Leucyl-tRNA synthetases (LeuRSs) are examples of aaRSs that rely on their editing domains to limit misaminoacylation of tRNA with near-cognate amino acids and maintain the fidelity of the genetic code. Here, we identified epetraborole (EPT) from the MMV pandemic response box as an inhibitor against the essential protein leucyl-tRNA synthetase (LeuRS) in M. abscessus. Benzoxaboroles were shown to inhibit LeuRS in fungi, gram-negative pathogens and most recently M. tuberculosis. To gain insight into the interactions between EPT and LeuRS, we solved the crystal structure of the M. abscessus editing domain (LeuRS303-498).

AMP acts as a surrogate for the 3’ end of the tRNA acceptor stem. In concordance with the binding mode of action of benzoxaboroles, we detected strong electron density in the active site corresponding to the EPT-AMP adduct formed through covalent interactions between the boron atom of EPT and the 2’ and 3’ hydroxyl groups on the ribose ring of AMP. In addition, R435 (R449 in M. tuberculosis) hydrogen bonds with the ethoxy oxygen of EPT and packed with the ribose of AMP. EPT has a hydroxypropyl ether moiety, rather than the ethyl ether in the benzoxaborole bound to M. tuberculosis LeuRS, but the extension shows very weak electron density and likely does not contribute to binding. The only notable difference is a ~1 Å shift in phosphate group of the EPT-AMP adduct. In both complexes, the phosphate is pinned between Y421 (Y435) and T323 (T337). The electron density indicates that there are multiple rotomeric conformations of T323, meaning its hydroxyl could hydrogen bond with the phosphate or with the 3’ O and ether oxygen of the adduct. Comparing unliganded and liganded residues in M. abscessus editing domain structures shows a sizable shift of residues 416–422, located around the adenosine pocket, upon drug binding, including ordering of Y421 to interact with the EPT-AMP adduct phosphate, and a decrease of B factors in the neighbouring residues. From the structural data, we propose that EPT binds LeuRS from M. abscessus and M. tuberculosis in a similar manner with similar affinity, providing a shared pathway for future structure-activity relationship analysis.

>SQGASVLFGAPGAGDIEVFTTRPDTLFGATYMVLAPEHPLVDQLAADVWPQDTDPRWTGGQDSPRAAIEQYRRSIAAKSDLERQENKEKTGVFTGAYATNPVSGKPVPVFIADYVLLGYGTGAIMAVPGHDQRDWDFANTFGLPVQEVISGGDVTKAAYTGDGVLVNSDYLDGLDIEAAKVEVTRRLVKDGRGESR[2x]> QFAKPEDAVKYRQSALTLMASHFGRMTPVVKGQAPYDAAQIKANVEVLKTLSALPWAAFGPGTEGG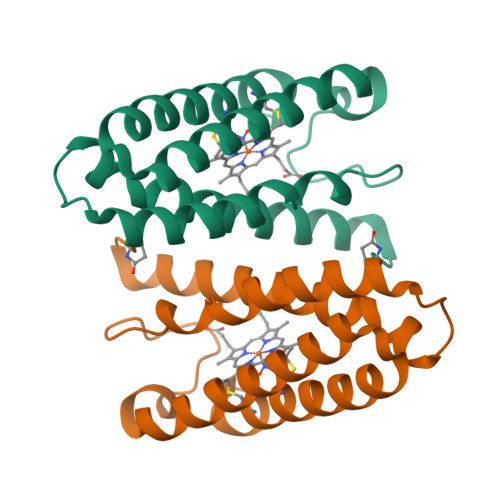DARPEIWSDAASFKQKQQAFQDNIVKLSAAADAGDLDKLRAAFGDVGASCKACHDAYEKKK NICOTINAMIDE ADENINE DINUCLEOTIDE CYCLOHEXANONE 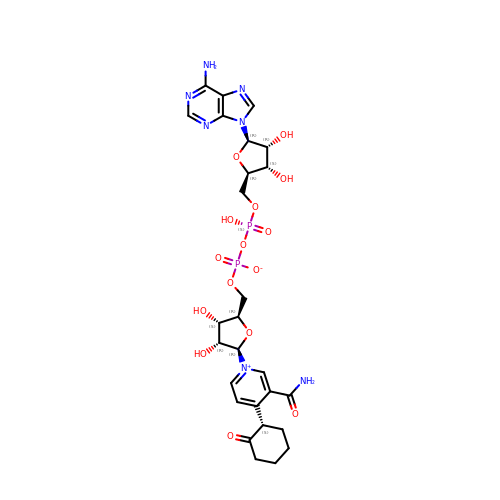| C27 H35 N7 O15 P2 | HTFHWJHTWKCYLR-RINXRSLZSA-N> GPGSEFMPKTISVRVTTMDAELEFAIQPNTTGKQLFDQVVKTIGLREVWFFGLQYQDTKAFSTWLKLNKKVTAQDVRKESPLLFKFRAKFYPEDVSEELIQDITQRLFFLQVKEGILNDDIYCPPETAVLLASYAVQSKYGDFNKEVHKSGYLAGDKLLPQRVLEQHKLNKDQWEERIQVWHEEHRGMLREDAVLEYLKIAQDLEMYGVNYFSIKNKKGSELWLGVDALGLNIYEQNDRLTPKIGFPWSEIRNISFNDKKFVIKPIDKKAPDFVFYAPRLRINKR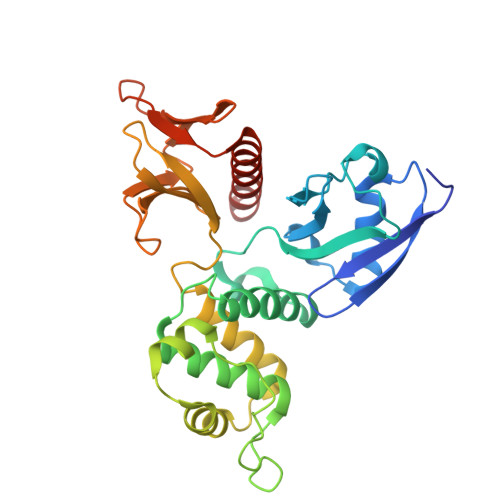ILALCMGNHELYMRRRKP> VTDSINWASGEDDHVVARAEYDF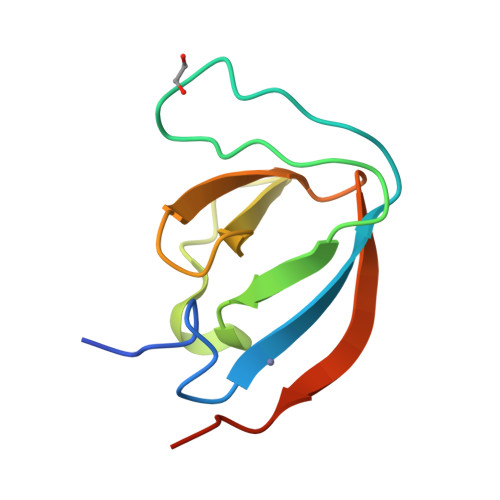AAVSEEEISFRAGDMLNLALKEQQPKVRGWLLASLDGQTTGLIPANYVKILGKRKGRKTVESS[(2~{R},3~{S},4~{R},5~{R})-5-(4-azanyl-2-oxidanylidene-pyrimidin-1-yl)-3,4-bis(oxidanyl)oxolan-2-yl]methyl ~{N}-[(2~{S})-2-azanyl-3-(4-hydroxyphenyl)propanoyl]sulfamate | C18 H23 N5 O9 S | 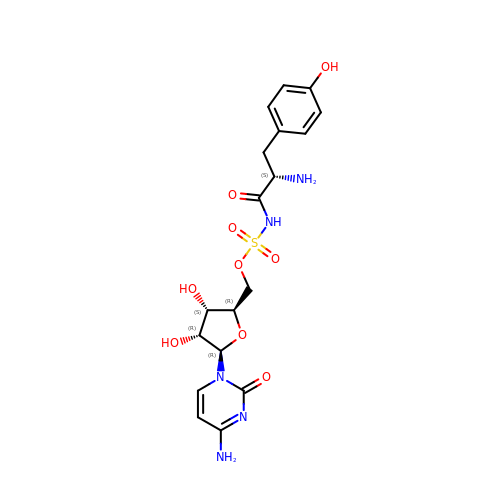CKVJPUGSXWTYBR-LMWHNAIISA-N> AGAAWACFRLDGRTLLRVRGPDAAPFLLGLLTNELPLPSPAAAGAPPAARAGYAHFLNVQGRTLYDVILYGLQEHSEVSGFLLECDSSVQGALQKHLALYRIRRKVTVEPHPELRVWAVLPSSPEACGAASLQERAGAAAILIRDPRTARMGWRLLTQDEGPALVPGGRLGDLWDYHQ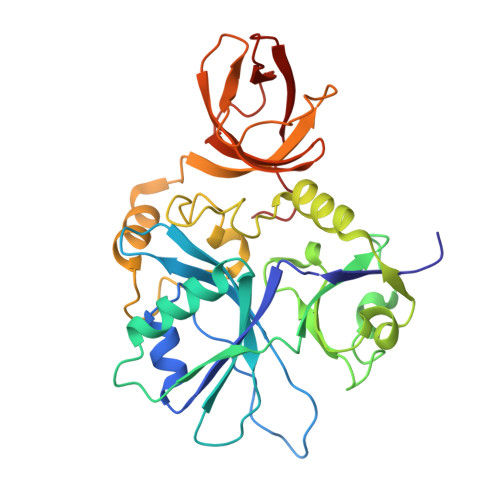HRYLQGVPEGVRDLPPGVALPLESNLAFMNGVSFTKGCYIGQELTARTHHMGVIRKRLFPVRFLDPLPTSGITPGATVLTASGQTVGKFRAGQGNVGLALLWSEKIKGPLHIRASEGAQVALAASVPDWWP> AETKIVVGPQPFSVGEEYPWLAERDEDGAVVTFTGKVRNHNLGDSVNALTLEHYPGMTEKALAE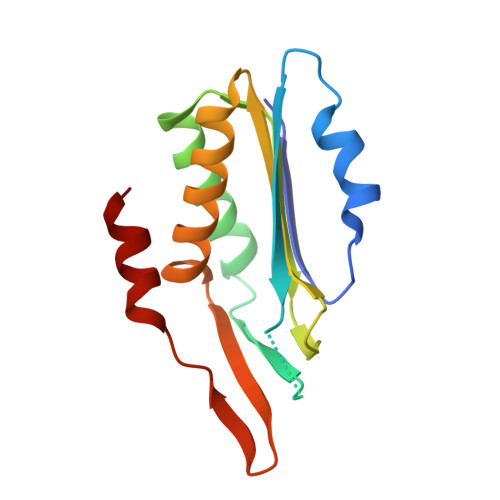IVDEARNRWPLGRVTVIHRIGELWPGDEIVFVGVTSAHRSSAFEAGQFIMDYLKTRAPFWKREATPEGDRWVEARESDQQAAKRW>[4x]MTADKLVFFVNGRKVVEKNADPETTLLAYLRRKLGLSGTKLGCGEGGCGACTVMLSKYDRLQNKIVHFSANACLAPICSLHHVAVTTVEGIGSTKTRLHPVQERIAKSHGSQCGFCTPGIVMSMYTLLRNQPEPTMEEIENAFQGNLCRCTGYRPILQGFRTFARDGGCCGGDGNNPNCCMNQKKDHSVSLSPSLFKPEEFTPLDPTQEPIFPPELLRLKDTPRKQLRFEGERVTWIQASTLKELLDLKAQHPDAKLVVGNTEIGIEMKFKNMLFPMIVCPAWIPELNSVEHGPDGISFGAACPLSIVEKTLVDAVAKLPAQKTEVFRGVLEQLRWFAGKQVKSVASVGGNIITASPISDLNPVFMASGAKLTLVSRGTRRTVQMDHTFFPGYRKTLLSPEEILLSIEIPYSREGEYFSAFKQASRREDDIAKVTSGMRVLFKPGTTEVQELALCYGGMANRTISALKTTQRQLSKLWKEELLQDVCAGLAEELHLPPDAPGGMVDFRCTLTLSFFFKFYLTVLQKLGQENLEDKCGKLDPTFASATLLFQKDPPADVQLFQEVPKGQSEEDMVGRPLPHLAADMQASGEAVYCDDIPRYENELSLRLVTSTRAHAKIKSIDTSEAKKVPGFVCFISADDVPGSNITGICNDETVFAKDKVTCVGHIIGAVVADTPEHTQRAAQGVKITYEELPAIITIEDAIKNNSFYGPELKIEKGDLKKGFSEADNVVSGEIYIGGQEHFYLETHCTIAVPKGEAGEMELFVSTQNTMKTQSFVAKMLGVPANRIVVRVKRMGGGFGGKETRSTVVSTAVALAAYKTGRPVRCMLDRDEDMLITGGRHPFLARYKVGFMKTGTVVALEVDHFSNVGNTQDLSQSIMERALFHMDNCYKIPNIRGTGRLCKTNLPSNTAFRGFGGPQGMLIAECWMSEVAVTCGMPAEEVRRKNLYKEGDLTH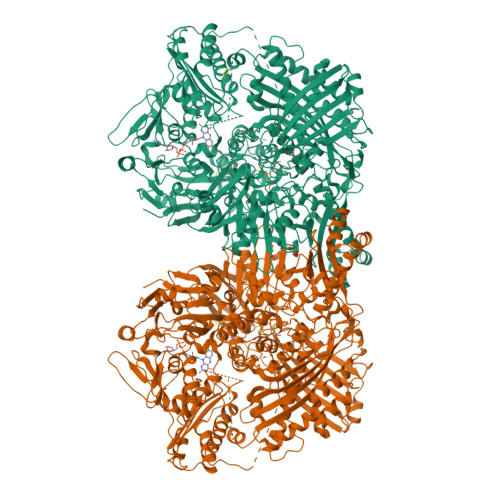FNQKLEGFTLPRCWEECLASSQYHARKSEVDKFNKENCWKKRGLCIIPTKFGISFTVPFLNQAGALLHVYTDGSVLLTHGGTEMGQGLHTKMVQVASRALKIPTSKIYISETSTNTVPNTSPTAASVSADLNGQAVYAACQTILKRLEPYKKKNPSGSWEDWVTAAYMDTVSLSATGFYRTPNLGYSFETNSGNPFHYFSYGVACSEVEIDCLTGDHKNLRTDIVMDVGSSLNPAIDIGQVEGAFVQGLGLFTLEELHYSPEGSLHTRGPSTYKIPAFGSIPIEFRVSLLRDCPNKKAIYASKAVGEPPLFLAASIFFAIKDAIRAARAQHTGNNVKELFRLDSPATPEKIRNACVDKFTTLCVTGVPENCKPWSVRV Adeno-associated virus (AAV) is a small ssDNA satellite virus of high interest (in recombinant form) as a safe and effective gene therapy vector. AAV’s human cell entry receptor (AAVR) contains polycystic kidney disease (PKD) domains bound by AAV. Seeking understanding of the spectrum of interactions, goat AAVGo.1 is investigated, because its host is the species most distant from human with reciprocal cross-species cell susceptibility. The AAV5 clade also includes AAVGo.1 (18, 19), which was isolated from deceased neonatal domesticated goat ileum.

Cryo-EM single particle analysis (SPA) yielded a reconstruction at 2.9 Å resolution for AAVGo.1. The structure of AAVGo.1, solved by cryo-EM to 2.9 Å resolution, is most similar to AAV5. The AAVGo.1 capsid has a similar protein fold and surface topology to AAV5 structures. The capsid core, comprising a jellyroll fold found in many virus structures, and a single α-helix (αA), is the most conserved feature of AAVs, and AAVGo.1 is no exception. The AAVGo.1 core jellyroll has the standard topology with a backbone chain alternating between two stacked antiparallel β-sheets (almost rolling into a single tube). AAVGo.1 and AAV5 capsid proteins have high homology (94%). DE loop (VR-II), which forms the outer edge of the pore-like structure of the 5-fold axis, protrudes an additional 1.5 Å compared to AAV5. A double serine insertion in VR-V of AAVGo.1 leads to two dislocations of 2.1 Å and 3.0 Å in the carbon backbone compared to AAV5. In conclusion, AAVGo.1 amino acid differences account for displacements up to 3.0 Å in VR-II and VR-V compared to the atomic structure of AAV5. AAVGo.1 residues Thr477 to Ser482 are of below-average order in the sharpened maps of AAVGo.1 alone.

> MSFVDHPPDWLEEVGEGLREFLGLEAGPPKPKPNQQHQDQARGLVLPGYNYLGPGNGLDRGEPVNRADEVAREHDISYNEQLEAGDNPYLKYNHADAEFQEKLADDTSFGGNLGKAVFQAKKRVLEPFGLVEEGAKTAPTGKRIDDHFPKRKKARTEEDSKPSTSSDAEAGPSGSQQLQIPAQPASSLGADTMSAGGGGPLGDNNQGADGVGNASGDWHCDSTWMGDRVVTKSTRTWVLPSYNNHQYREIKSGSVDGSNANAYFGYSTPWGYFDFNRFHSHWSPRDWQRLINNYWGFRPRSLRVKIFNIQVKEVTVQDSTTTIANNLTSTVQVFTDDDYQLPYVVGNGTEGCLPAFPPQVFTLPQYGYATLNRDNGDNPTERSSFFCLEYFPSKMLRTGNNFEFTYSFEEVPFHCSFAPSQNLFKLANPLVDQYLYRFVSTSATGAIQFQKNLAGRYANTYKNWFPGPMGRTQGWNTSSGSSTNRVSVNNFSVSNRMNLEGASYQVNPQPNGMTNTLQGSNRYALENTMIFNAQNATPGTTSVYPEDNLLLTSESETQPVNRVAYNTGGQMATNAQNATTAPTVGTYNLQEVLPGSVWMERDVYLQGPIWAKIPETGAHFHPSPAMGGFGLKHPPPMMLIKNTPVPGNITSFSDVPVSSFITQYSTGQVTVEMEWELKKENSKRWNPEIQYTNNYNDPQFVDFAPDGSGEYRTTRAIGTRYLTRPL> LQQWKVGDKCSAIWSEDGCIYPATIASIDFKRETCVVVYTGYGN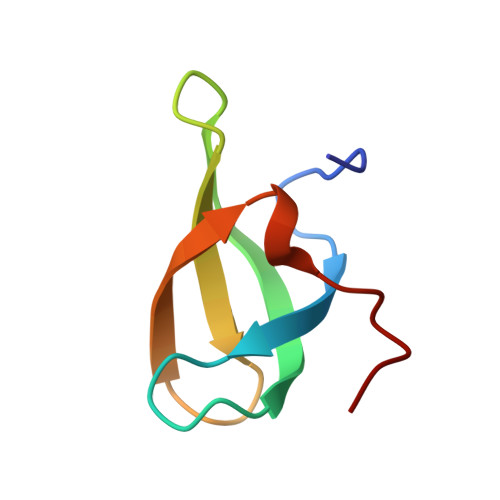REEQNLSDLLSPICE> GPLVPESLQEQIQSNFIIVIHPGSTTLRIGRATDTLPASIPHVIARRHKQQGQPLYKDSWLLREGLNKPESNEQRQNGLKMVDQAIWSKKMSNGTRRIPVSPEQARSYNKQMRPAILDHCSGNKWTNTSHHPEYLVGEEALYVNPLDCYNIHWPIRRGQLNIHPGPGGSLTAVLADIEVIWSHAIQKYLEIPLKDLKYYRCILLIPDIYNKQHVKELVNMILMKMGFSGIVVHQESVCATYGSGLSSTCIVDVGDQKTSVCCVEDGVSHRNTRLCLAYGGSDVSRCFYWLMQRAGFPYRECQLTNKMDCLLLQHLKETFCHLDQDISGLQDHEFQIRHPDSPALLYQFRLGDEKLQAPMALFYPATFGIVGQKMTTLQHRSQGDPEDPHDEHYLLATQSKQEQSAKATADRKSASKPIGFEGDLRGQSSDLPERLHSQEVDLGSAQGDGLMAGNDSEEALTALMSRKTAISLFEGKALGLDKAILHSIDCCSSDDTKKKMYSSILVVGGGLMFHKAQEFLQHRILNKMPPSFRRIIENVDVITRPKDMDPRLIAWKGGAVLACLDTTQELWIYQREWQRFGVRMLRERAAFVW

A notable, poorly understood feature of several large multi-subunit chromatin modifying or remodeling complexes is the presence of nuclear actin-related proteins (Arps) (1) along with nuclear actin (2). INO80 contains actin along with Arp4, Arp5 and Arp8. Actin, Arp4 and Arp8 together with the helicase-SANT-associated (HSA) domain of the Ino80 ATPase form a stable sub-module of INO80 (9), while Arp5 together with INO80 subunits Ies2 and Ies6 associate with the AAA+ ATPase subunits Rvb1/Tip49 and Rvb2/Tip48 (10). Deleting Arp8 in Saccharomyces cerevisiae results in an INO80 complex that also lacks Arp4 and actin, in addition to the losses of DNA binding and ATPase activities.

To provide a first structural framework for Arp8 we determined the crystal structure of Homo sapiens Arp8 (a truncated variant that lacks the first 33 N-terminal amino acids), and studied the solution structure of truncated and full-length human Arp8 (hArp8) by small angle X-ray scattering (SAXS). The crystals contained one Arp8 molecule per asymmetric unit. Except for 91 amino acids (R411–I501) in a loop insertion, we obtained interpretable electron density for the entire protein. Additional density in the nucleotide-binding cleft could be interpreted as a bound ATP molecule with one coordinated metal ion. Since ATP was not added prior to crystallization, it was retained from the cells throughout purification and crystal growth. Despite the relatively low sequence homology to actin, human Arp8 displays the typical actin fold with a central nucleotide-binding cleft between sub-domains 1 and 2 on one side and sub-domains 3 and 4 on the other side. The most notable feature of Arp8 is a long insertion I (K80–H162), which emanates from the ‘DNaseI binding loop’ (D-loop) on sub-domain 2, binds across both halves of the actin fold to wrap around sub-domain 4 and reaches back to the D-loop. All in all, insertions I–III appear to lock the two principal domains of actin (sub-domains 1–2 and sub-domains 3–4) into a particular conformation and stabilize the active site cleft. While the concave side only carries small insertions, the Arp8 characteristic insertions cover the convex (filament facing side of actin) and pointed side of the molecule and explain why Arp8 itself does not form filaments. On the contrary, the nucleotide-binding site of Arp8 exhibits only minor changes to the residues involved in the catalytic cycle of actin’s ATPase.> MNRPAPVEVTYKNMRFLITHNPTNATLNKFIEELKKYGVTTIVRVCEATYDTTLVEKEGIHVLDWPFDDGAPPSNQIVDDWLSLVKIKFREEPGCCIAVHCVAGLGRAPVLVALALIEGGMKYED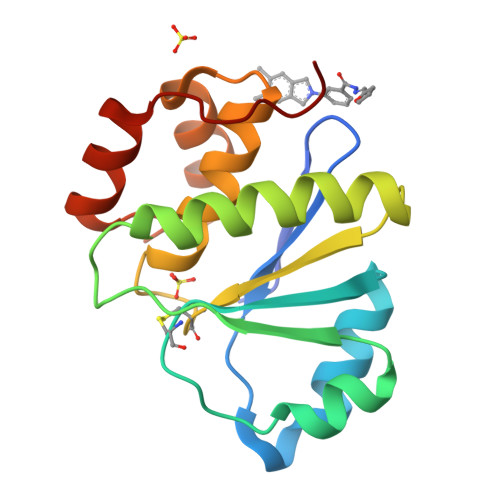AVQFIRQKRRGAFNSKQLLYLEKYRPKMRLRF>MSSTPSNQNIIPIIKKESIVSLFEKGIRQDGRKLTDYRPLSITLDYAKKADGSALVKLGTTMVLAGTKLEIDKPYEDTPNQGNLIVNVELLPLAYTTFEPGPPDENAIELARVVDRSLRDSKALDLTKLVIEPGKSVWTVWLDVYVLDYGGNVLDACTLASVAALYNTKVYKVEQISVNKNEVVGKLPLNYPVVTISVAKVDKYLVVDPDLDEESIMDAKISFSYTPDLKIVGIQKSGKGSMSLQDIDQAENTARSTAVKLLEELKKHLGI[3x];>MLQVERPKLILDDGKRTDGRKPDELRSIKIELGVLKNADGSAIFEMGNTKAIAAVYGPKEMHPRHLSLPDRAVLRVRYHMTPFSTDERKNPAPSRREIELSKVIREALESAVLVELFPRTAIDVFTEILQADAGSRLVSLMAASLALADAGIPMRDLIAGVAVGKADGVIILDLNETEDMWGEADMPIAMMPSLNQVTLFQLNGSMTPDEFRQAFDLAVKGINIIYNLEREALKSKYVEFKEEG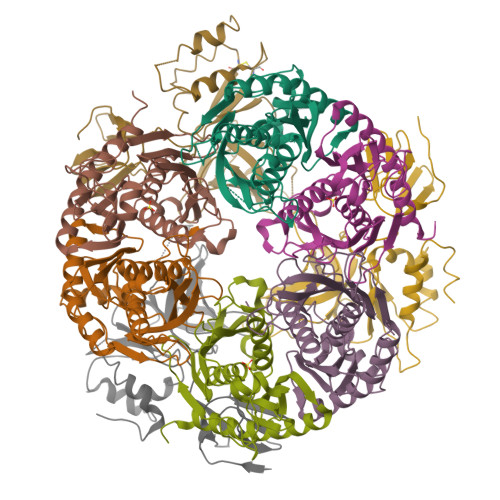V[3x];>MNMSQSQKIVLQPRSIVVPGELLAEGEFQIPWSPYILKINSKYYSTVVGLFDVKDTQFEVIPLEGSFYYPKINDIVIGLVEDVEIYGWVVDIKAPYKAYLPASNLLGRSINVGEDLRRYLDVGDYVIARIENFDRSIDPVLSVKGKDLGRVSNGIVIDIMPVKVPRVIGKNKSMYETLTSKSGCSIFVANNGRIWATCPSRFSEEILIEAIRKIENESHIKGLTDRIKQFIEEKLGERNASSGETKTNS[3x]> YNISEMRIIGDTQKLDNELNQLLTHFKAGQLFRKTELSIIEEQIKQILGDRGYGSAKVDLYPKFNEEDHTVQINFIVDA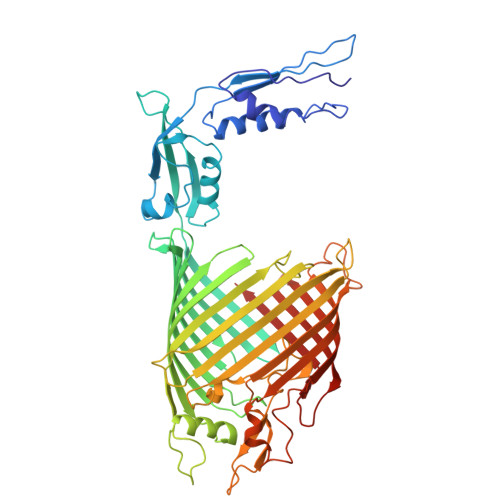GRRIYVRKIRFEGNDVTADSTLRREMRQQEGAWLSTSAVSLAKSRLERTGFYETVEMSMPTVKNTDDQVDIIYKIKERNTGSINFGVGYGSGSGLSYNAGITQDNFLGMGSSLGLNGSRNTDSTNVNLSYTEPYFTKDGVSLGGNIFYEDYDNSARKASAAYKRKTYGASGTLGFPVDENNSYYLGLGYTHDKLRNVEREYTREKYVNSMKFPINPQNSHYDRIQSADFDLSFGWNYNNLNRGYFPTAGSSANISGKLTLPGSDNKYYQVGTNFSGYIPLNSEHKWVIATKGGLAYTNSFGGKEVPFYQLYSAGGMGSLRGFAGGSIGPKAIYYREDGFKAPSQDVIGGNAMVNASLELIIPAPFISDKYQHNVRTSVFVDAATVWNTKWKQSKADYPNLPDFGDYKRVRASAGIALQWQSPIGPLSFSYAKPIKKYAGDEIEQFQFTVGSTF> ATPADWRSQSIYFLLTDRFARTDGSTTATCNTADQKYCGGTWQGIIDKLDYIQGMGFT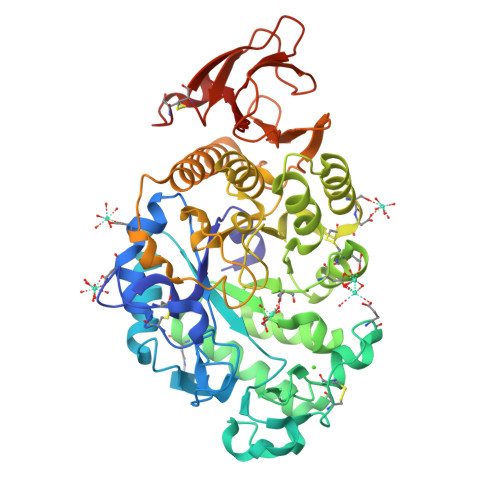AIWITPVTAQLPQTTAYGDAYHGYWQQDIYSLNENYGTADDLKALSSALHERGMYLMVDVVANHMGYDGAGSSVDYSVFKPFSSQDYFHPFCFIQNYEDQTQVEDCWLGDNTVSLPDLDTTKDVVKNEWYDWVGSLVSNYSIDGLRIDTVKHVQKDFWPGYNKAAGVYCIGEVLDGDPAYTCPYQNVMDGVLNYPIYYPLLNAFKSTSGSMDDLYNMINTVKSDCPDSTLLGTFVENHDNPRFASYTNDIALAKNVAAFIILNDGIPIIYAGQEQHYAGGNDPANREATWLSGYPTDSELYKLIASANAIRNYAISKDTGFVTYKNWPIYKDDTTIAMRKGTDGSQIVTILSNKGASGDSYTLSLSGAGYTAGQQLTEVIGCTTVTVGSDGNVPVPMAGGLPRVLYPTEKLAGSKICSSS>[2x]MGHHHHHHGDAALLLNVEGVKKTILHGGTGELPNFITGSRVIFHFRTMKCDEERTVIDDSRQVGQPMHIIIGNMFKLEVWEILLTSMRVHEVAEFWCDTIH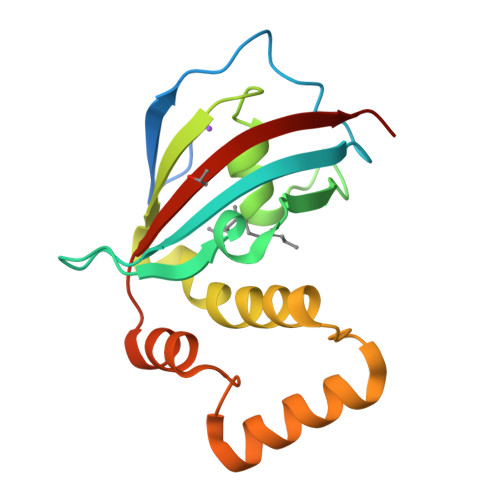TGVYPILSRSLRQMAQGKDPTEWHVHTCGLANMFAYHTLGYEDLDELQKEPQPLVFVIELLQVDAPSD> MKVIFLKDVKGKGKKGEIKN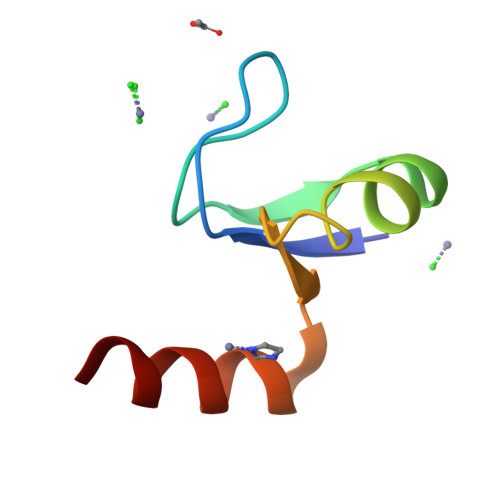VADGYANNFLFKQALAIEATPANLKALEAQKQ(2R)-(3-chlorophenyl)(hydroxy)ethanoic 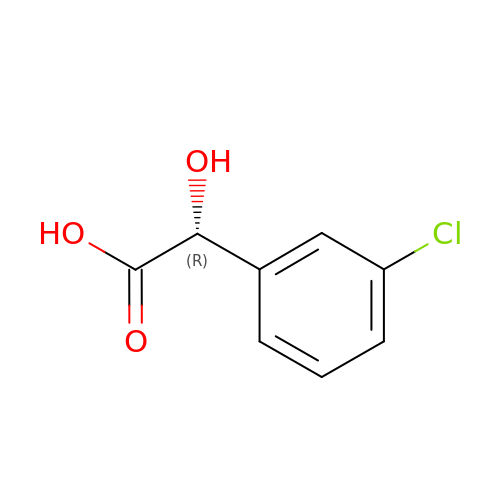acid | C8 H7 Cl O3 | SAMVPMGKGGLIPF-SSDOTTSWSA-N In the CU pathway, a dedicated chaperone facilitates the folding of pilus subunits in the periplasm and an integral outer membrane (OM) protein termed the usher provides the assembly platform and secretion channel for the pilus fiber. Periplasmic chaperone–subunit complexes are then recruited to the OM usher (PapC for P pili, FimD for type 1 pili) for subunit assembly into pili and secretion of the pilus fiber to the cell surface. Ushers contain five domains: a central 24-stranded ß-barrel domain that inserts into the OM to form the secretion channel, an internal plug domain that forms the channel gate, a periplasmic N-terminal domain (NTD) that functions in subunit recruitment, and two tandem periplasmic C-terminal domains (CTD1 and CTD2) that function in pilus assembly and secretion. Using cryo-electron microscopy (EM), we determined structures of the activated PapC usher in the process of secreting two- and three-subunit P pilus assembly intermediates.

To generate a two-subunit intermediate, we replaced the PapK NTE with the NTE from PapF (PapKF-NTE) and deleted papE and papF, resulting in a ∆EF P pilus tip fiber composed only of PapK bound to PapG. For the two-subunit ∆EF dataset, starting with over one million particles, after 2D and 3D classifications, we derived two 3D maps, named Conformers II and III, at 3.8 Å and 7.2 Å, respectively. In the ∆EF cryo-EM structures (Conformers II and III), the PapF subunit is not present and instead PapK is directly engaged in DSE (by its engineered PapF NTE) with the pilin domain of PapG. The lectin domain of PapG in Conformers II and III has not yet fully transited through the usher channel and the PapG pilin domain is still located on the periplasmic side of the usher. In Conformers II and III, the PapC plug domain, NTD, and CTDs are resolved in the 3D maps and reside on the periplasmic side of the β-barrel channel. In the Conformer II ∆EF structure, the usher NTD is bound to the N-terminal end of the first lobe of PapD, as in Conformer I, but here CTD2 of the PapC usher is visible. CTD2 is bound to PapD in a never-before-seen binding site at the vertex of the boomerang, where CTD2 primarily interacts with the C-terminal end of the first lobe of PapD. Due to this binding and stabilization of CTD2, we propose that Conformer II follows Conformer I in the chaperone–subunit recruitment and handover cycle that takes place on the periplasmic domains of the usher. The interactions between PapC CTD2 and PapD are more complicated: in Conformer II, F732 and W767 of CTD2 interact hydrophobically with A119 and I120 of PapD, respectively; in Conformer III, F732 and W767 of CTD2 form hydrophobic interactions with I46, I51, and P73 of PapD. (4) Next, the handover of PapDF from the NTD to the CTDs is initiated by binding of CTD2 to the midpoint of the PapD chaperone (Conformer II).

> VEFNTDVLDAADKKNIDFTRFSEAGYVLPGQYLLDVIVNGQSISPASLQISFVEPQSSGDKAEKKLPQACLTSDMVRLMGLTAESLDKVVYWHDGQCADFHGLPGVDIRPDTGAGVLRINMPQARLEYSDATWLPPSRWDDGIPGLMLDYNLNGTVSRNYQGGDSHQFSYNGTVGGNLGPWRLRADYQGSQEQSRYNGEKTTNRNFTWSRFYLFRAIPRWRANLTLGENNINSDIFRSWSYTGASLESDDRMLPPRLRGYAPQITGIAETNARVVVSQQGRVLYDSMVPAGPFSIQDLDSSVRGRLDVEVIEQNGRKKTFQVDTASVPYLTRPGQVRYKLVSGRSRGYGHETEGPVFATGEASWGLSNQWSLYGGAVLAGDYNALAAGAGWDLGVPGTLSADITQSVARIEGERTFQGKSWRLSYSKRFDNADADITFAGYRFSERNYMTMEQYLNARYRNDYSSREKEMYTVTLNKNVADWNTSFNLQYSRQTYWDIRKTDYYTVSVNRYFNVFGLQGVAVGLSASRSKYLGRDNDSAYLRISVPLGTGTASYSGSMSNDRYVNMAGYTDTFNDGLDSYSLNAGLNSGGGLTSQRQINAYYSHRSPLANLSANIASLQKGYTSFGVSASGGATITGKDAALHAGGMSGGTRLLVDTDGVGGVPVDGGQVVTNRWGTGVVTDISSYYRNTTSVDLKRLPDDVEATRSVVESALTEGAIGYRKFSVLKGKRLFAILRLADGSQPPFGASVTSEKGRELGMVADEGLAWLSGVTPGETLSVNWDGKIQCQVNVPETAISDQQLLLPCTPQK;> MIRKKILMAAIPLFVISGADAAVSLDRTRAVFDGSEKSMTLDISNDNKQLPYLAQAWIENENQEKIITGPVIATPPVQRLEPGAKSMVRLSTTPDISKLPQDRESLFYFNLREIPPRSEKANVLQIALQTKIKLFYRPAAIKTRPNEVWQDQLILNKVSGGYRIENPTPYYVTVIGLGGSEKQAEEGEFETVMLSPRSEQTVKSANYNTPYLSYINDYGGRPVLSFICNGSRCSVKKEK;> MKKWFPALLFSLCVSGESSAWNNIVFYSLGDVNSYQGGNVVITQRPQFITSWRPGIATVTWNQCNGPGFADGFWAYYREYIAWVVFPKKVMTQNGYPLFIEVHNKGSWSEENTGDNDSYFFLKGYKWDERAFDAGNLCQKPGETTRLTEKFDDIIFKVALPADLPLGDYSVKIPYTSGMQRHFASYLGARFKIPYNVAKTLPRENEMLFLFKNIGGCRPSAQSLEIKHGDLSINSANNHYAAQTLSVSCDVPANIRFMLLRNTTPTYSHGKKFSVGLGHGWDSIVSVNGVDTGETTMRWYKAGTQNLTIGSRLYGESSKIQPGVLSGSATLLMILP;> MIKSTGALLLFAALSAGQAIASDVAFRGNLLDRPCHVSGDSLNKHVVFKTRASRDFWYPPGRSPTESFVIRLENCHATAVGKIVTLTFKGTEEAALPGHLKVTGVNAGRLGIALLDTDGSSLLKPGTSHNKGQGEKVTGNSLELPFGAYVVATPEALRTKSVVPGDYEATATFELTYR> ETGSAQQLNEDLRLHLLLNTSVTCNDGSPAGYYLKESRGSRRWLLFLEGGWYCFNRENCDSRYDTMRRLMSSRDWPRTRTGTGILSSQPEENPYWWNANMVFIPYCSSDVWSGASSKSEKNEYAFMGALIIQEVVRELLGRGLSGAKVLLLAGSAAGGTGVLLNVDRVAEQLEKLGYPAIQVRGLADSGWFLDNKQYRHTDCVDTITCAPTEAIRRGIRYWNGVVPERCRRQFQEGEEWNCFFGYKVYPTLRSPVFVVQWLFDEAQLTVDNVHLTGQPVQEGLRLYIQNLGRELRHTLKDVPASFAPACLSHEIIIRSHWTDVQVKGTSLPRALHCWDRSLHDSHKASKTPLKGCPVHLVDSCPWPHCNPSC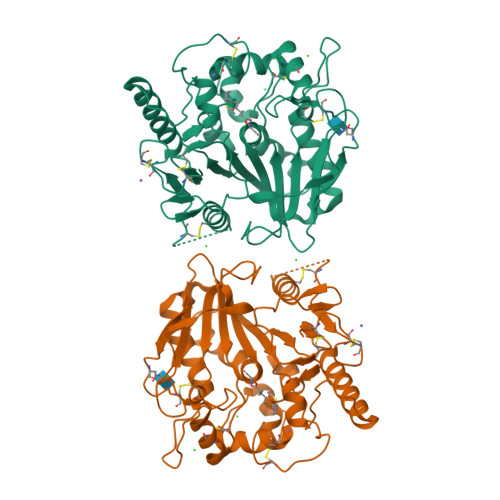PTGTHHHHHHHHHH;> CHGVSGSC> GSMIVTQTHRAISQVVKQAK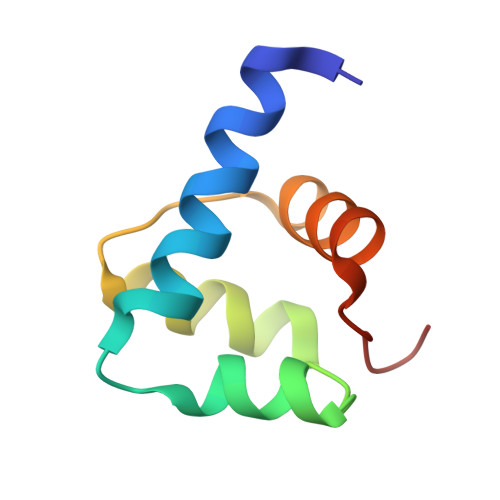DNSVWIKILTYSAIDVEEFQLWLKRKNLNVSLDLIKSWCDKYGVLMKGSWH>[4x]GSHMEPPPKLVLDLERMAHVPQEKAGP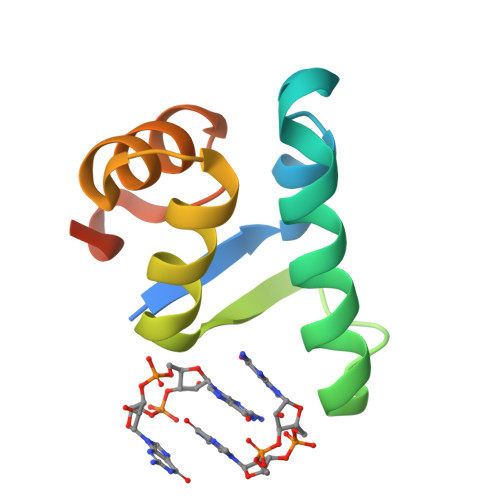LQRYAATIQSQRGDYNGKVLSIRQDDLRTLAVIYDQSPSVLTEQLISWGVLDADARRAVAHEEN> MEHVAFGSEDIENTLAKMDDGQLDGLAFGAIQLDG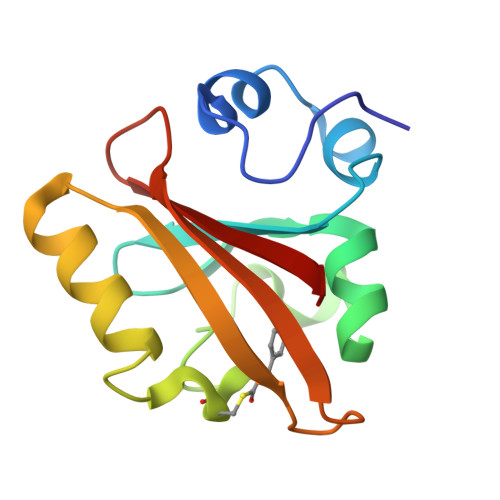DGNILQYNAAEGDIVGRDPKQVIGKNFFKDVAPCTDSPEFYGKFKEGVASGNLNTMFEYTFDYQMTPTKVKVHMKKALSGDSYWVFVKRV> MAAKRYTSMAYANADEMTFGVSKYPVKAGLDLEIGAGYTIPEINYAPRPEAGASKEKLIKEYERITTDVMERMVQVGFPAIILETEHVQQMSNNPSWGAEVAHAQKTIMEKYHDEYGIKCALRHTIGDIRENREFLQLRGDKYSVFLEAFEQCAENGADLLSVESMGGKEVFDYAVLRNDIPGLLYSIGCLGSIDMELIWTDISKIAKK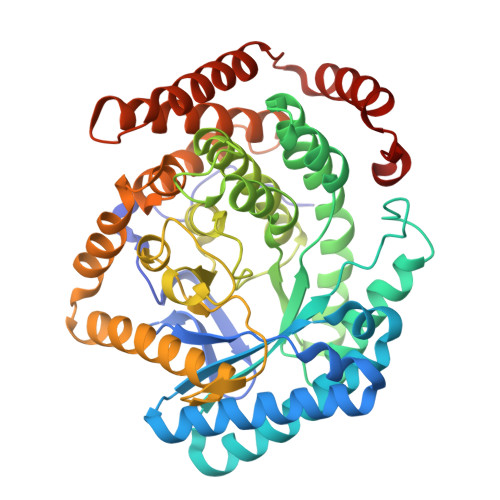TGTISAGDTDCAQANTAMFIGGGLLNKNLAHTIAVIARAISAPRSLVAYEAGAVGPGKDCGYENIIVKAITGMPMTMEGKTSTCAHSDVMGNLVMQCCDCWSNESVEYHGEFGGTTVQCWSETLAYDCALMNTALETKNDKVLRDLMMLSDRYRDPQAYMLAYDNAYRVGQSIVKDGDNIYLRAKNAAIECCNIIEEGAAGKLELSRFETKALADAKAALEALPDDMDKFMDDCLTKYKSEVKVFKPENYGF>[2x]MNPAAEAEFNILLATDSYKVTHYKQYPPNTSKVYSYFECREKKTENSKLRKVKYEETVFYGLQYILNKYLKGKVVTKEKIQEAKD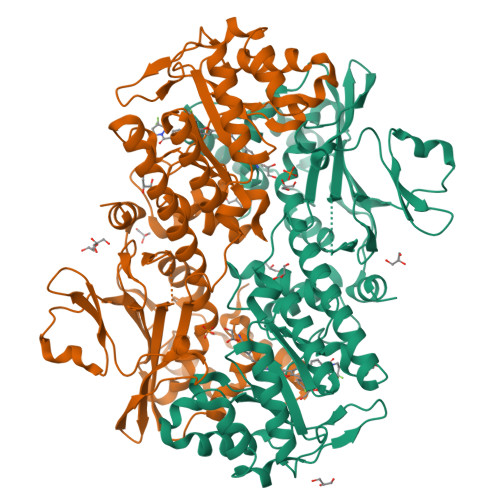VYKEHFQDDVFNEKGWNYILEKYDGHLPIEIKAVPEGFVIPRGNVLFTVENTDPECYWLTNWIETILVQSWYPITVATNSREQKKILAKYLLETSGNLDGLEYKLHDFGYRGVSSQETAGIGASAHLVNFKGTDTVAGLALIKKYYGTKDPVPGYSVPAAEHSTITAWGKDHEKDAFEHIVTQFSSVPVSVVSDSYDIYNACEKIWGEDLRHLIVSRSTQAPLIIRPDSGNPLDTVLKVLEILGKKFPVTENSKGYKLLPPYLRVIQGDGVDINTLQEIVEGMKQKMWSIENIAFGSGGGLLQKLTRDLLNCSFKCSYVVTNGLGINVFKDPVADPNKRSKKGRLSLHRTPAGNFVTLEEGKGDLEEYGQDLLHTVFKNGKVTKSYSFDEIRKNAQLNIELEAAHHENLYFQ>[3x]MVNNNRPRRQRAQRVVVTTTQTAPVPQQNVPRNGRRRRNRTRRNRRRVRGMNMAALTRLSQPGLAFLKCAFAPPDFNTDPGKGIPDRFEGKVVSRKDVLN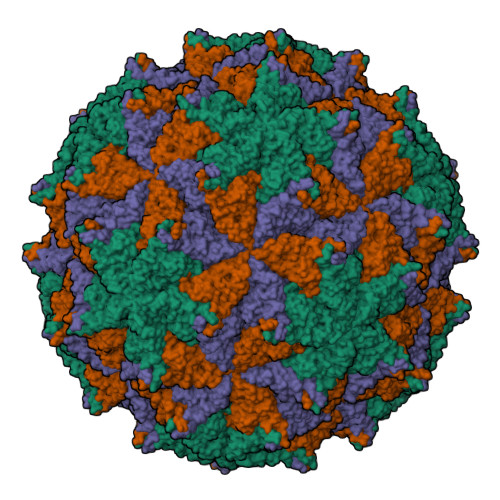QSISFTAGQDTFILIAPTPGVAYWSASVPAGTFPTSATTFNPVNYPGFTSMFGTTSTSRSDQVSSFRYASMNVGIYPTSNLMQFAGSITVWKCPVKLSTVQFPVATDPATSSLVHTLVGLDGVLAVGPDNFSESFIKGVFSQSACNEPDFEFNDILEGIQTLPPANVSLGSTGQPFTMDSGAEATSGVVGWGNMDTIVIRVSAPEGAVNSAILKAWSCIEYRPNPNAMLYQFGHDSPPLDEVALQEYRTVARSLPVAVIAAQN>[2x]SLFE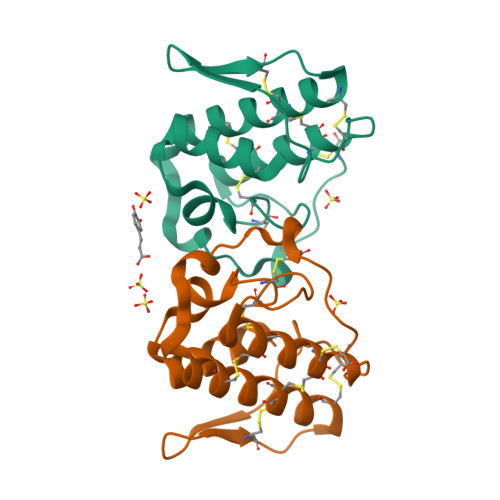LGKMILQETGKNPAKSYGAYGCNCGVLGRGQPKDATDRCCYVHKCCYKKLTGCDPKKDRYSYSWKDKTIVCGENNPCLKELCECDKAVAICLRENLGTYNKKYRYHLKPFCKKADPC>[2x]GHMWQENKSWNAHFTEHKSQGVVVLWNENKQQGFTNNLKRANQAFLPASTFAIPNSLIALDLGVVKDEHQVFKWDGQTRDIATW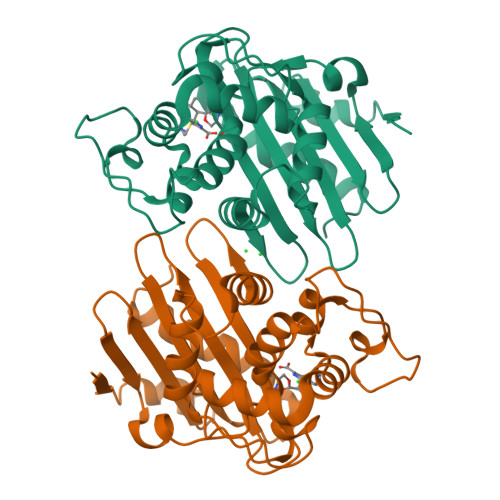NRDHNLITAMKYSVVPVYQEFARQIGEARMSKMLHAFDYGNEDISGNVDSFWLDGGIRISATEQISFLRKLYHNKLHVSERSQRIVKQAMLTEANGDYIIRAKTGYSTRIEPKIGWWVGWVELDDNVWFFAMNMDMPTSDGLGLRQAITKEVLKQEKIIP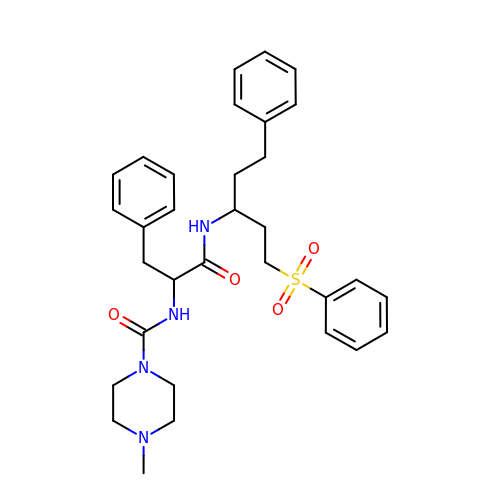NALPHA-[(4-METHYLPIPERAZIN-1-YL)CARBONYL]-N-{(1S)-3-PHENYL-1-[2-(PHENYLSULFONYL)ETHYL]PROPYL}-L-PHENYLALANINAMIDE | C32 H40 N4 O4 S | VZSXPUDQSLKVIR-JDXGNMNLSA-N>MKEIKLILTDIDGVWTDGGMFYDQTGNEWKKFNTSDSAGIFWAHNKGIPVGILTGEKTEIVRRRAEKLKVDYLFQGVVDKLSAAEELCNELGINLEQVAYIGDDLN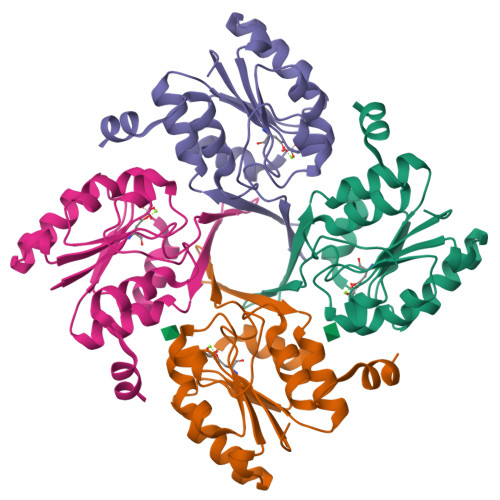DAKLLKRVGIAGVPASAPFYIRRLSTIFLEKRGGEGVFREFVEKVLGINLEDFIAVIQ[4x]> MGSSHHHHHHSQDPDQVQYENTLKNF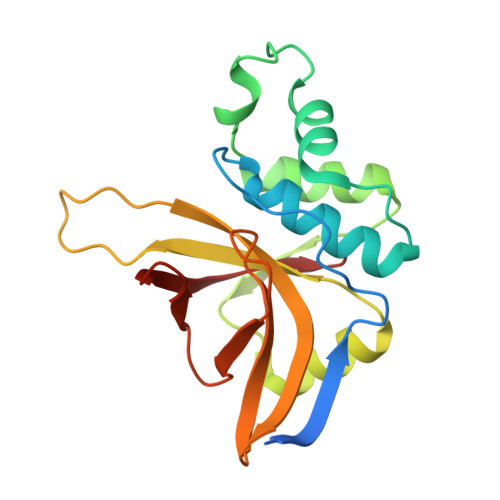KIREQQFDNSWCAGFSMAALLNATKNTDTYNAHDIMRTLYPEVSEQDLPNCATFPNQMIEYGKSQGRDIHYQEGVPSYNQVDQLTKDNVGIMILAQSVSQNPNDPHLGHALAVVGNAKINDQEKLIYWNPWDTELSIQDADSSLLHLSFNRDYNWYGSMIGY> PLDPRIKKLLESGFVVPIGKASVDEVRKIFRQLASAAPKAEVRKVEDIKIPGSETSINARVYFPKAKGPYGVLVYLHGGGFVIGDVESYDPLCRAITNACNCVVVSVDYRLAPEYKFPSAVIDSFDATNWIYNNLDKFDGEMGIAIAGDSAGGNLAAVVALLSKGKLDLKYQILIYPAVGFDSVSRSMIEYSDGFFLTREHIEWFGSQYLRSPADLLDFRFSPIIAQDLSGLPPA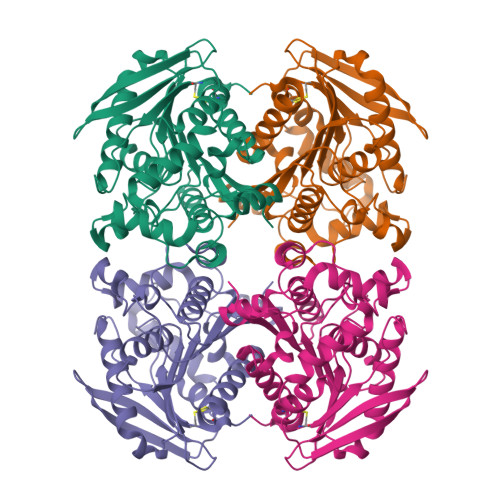LIITAEYDPLRDPEEAYANRLLQAGVPVTSVRFNNVIHGFLSFFPLIDQGKDAIGLIGSVLRRTFYDKS Matrix protein (MA), p15 in FIV or EIAV and p17 in HIV or SIV, is the N-terminal subunit of the retroviral Gag polyprotein. During the viral replication cycle, the FIV p15 matrix protein oligomerizes to form a closed matrix that underlies the lipidic envelope of the virion. In FIV, HIV or SIV, the N-terminal domain of Gag undergoes a co-translational covalent modification of the MA N-terminus with a myristoyl group. This myristoylation, together with a highly basic patch of amino acid residues located at the N-terminus of the MA, directs the Gag polyprotein to the plasma membrane (PM), mediating the association between Gag and the inner leaflet of the PM lipid bilayer, where Gag forms a hexagonal network. The structure consists of five α-helices (numbered h1 to h5 following the HIV convention), which give rise to the close packing of adjacent helices typical for retroviral matrix proteins.

To investigate which interface could be the biological dimer that we observe in vitro, we constructed a shortened form of FIV p15, p15-Δ120, which is truncated after Ser120 to remove the residues involved in interface 1. The p15-Δ120 truncated protein was stable and was still able to generate dimers in solution in MES buffer, even at a lower protein concentration (3 mg/ml). Crystals of p15-Δ120 could be grown, and data could be collected to 2.6 Å resolution. The crystal space group for p15-Δ120 is different (P21) from the full-length protein (P21212), and 2 monomers are present in the asymmetric unit. The truncation of the last 14 residues does not alter the overall conformation of the protein, as demonstrated by the RMSD of 0.5 Å between the Cα pairs in the truncated protein and the full-length protein. The assembly in the asymmetric unit of p15-Δ120 resembled the interface 2 observed with the full-length protein. As expected, interface 1 is no longer present in the crystal packing of p15-Δ120 as the C-terminal residues involved in this interface with the full-length protein were truncated. However, Trp37, which was involved in the hydrophobic interaction with Pro131 in interface 1, is not free in the p15-Δ120 crystal. Instead, this conserved residue demonstrates hydrophobic interactions with a PEG fragment from the crystallization solution in both monomers of the asymmetric unit. Finally, the interface 3 observed in the full-length protein is maintained in the crystal packing of p15-Δ120 with a similar buried surface and intermolecular interactions as the full-length protein.

>[2x]MGNGQGRDWKMAIKRCSNVAVGVGGKSKKFGEGNFRWAIRMANVSTGREPGDIPETLDQLRLVICDLQERREKFGSSKEIDMAIVTLKVFAVAGLLNMTVSTAAAAENMYSQMGLDTRPSLVPRGSLEHHHHHH2-[(3-Nitro-2-pyridyl)thio]acetic acid | C7 H6 N2 O4 S | 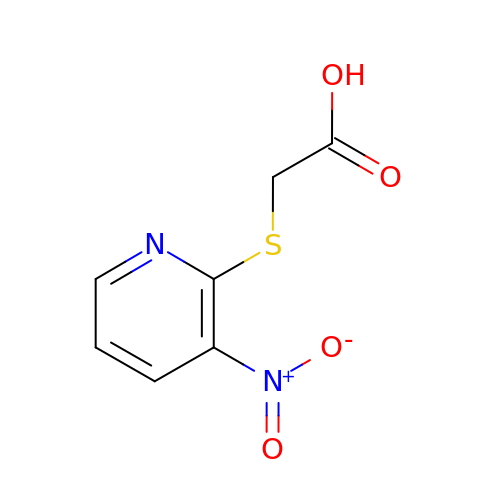WBPUHBNGHSAAGT-UHFFFAOYSA-N> LPFELRG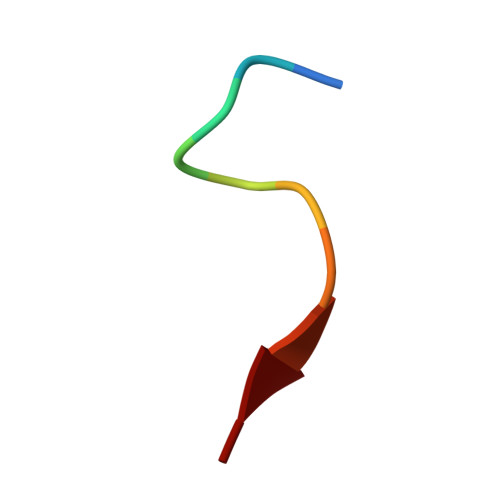HLV(2R)-2-hydroxy-4-methylpentanoic acid | C6 H12 O3 | 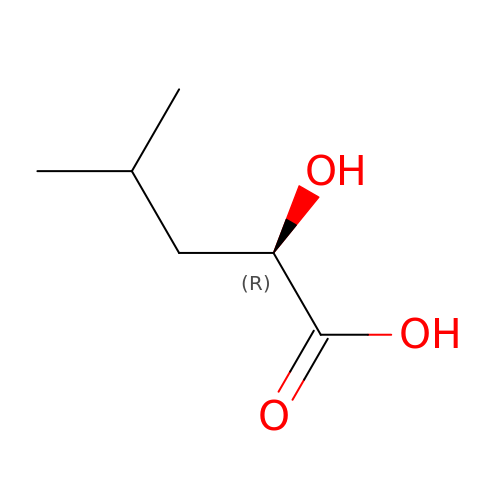LVRFTAZAXQPQHI-RXMQYKEDSA-N>MASQTITVGPWGGSGGNGWDDGSYTGIRQIELSYKEAIGSFCVIYDLNGESFPGPKHTSKLPYKNVKIELQFPEEFLVSVSGYTGPFSALATPTPVVRSLTFKTNKGRTFGPYGDEEGTYFNLPIENGLIVG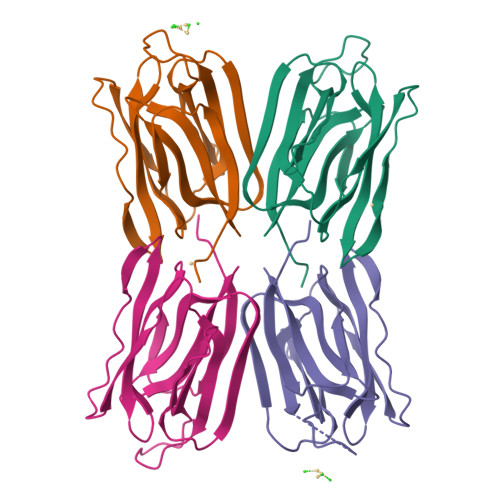FKGRTGDLLDAIGVHMAL[4x]>[2x]MTT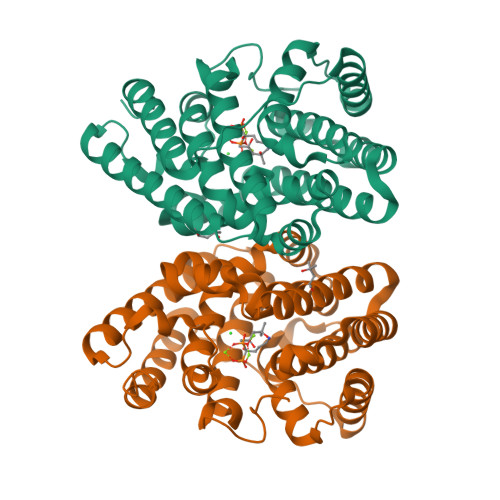GLSTAGAQDIGRSSVRPYLEECTRRFQEMFDRHVVTRPTKVELTDAELREVIDDCNAAVAPLGKTVSDERWISYVGVVLWSQSPRHIKDMEAFKAVCVLNCVTAVWDDMDPALHDFGLFLPQLRKICEKYYGPEDAEVAYEAARAFVTSDHMFRDSPIKAALCTTSPEQYFRFRVTDIGVDFWMKMSYPIYRHPEFTEHAKTSLAARMTTRGLTIVNDFYSYDREVSLGQITNCFRLCDVSDETAFKEFFQARLDDMIEDIECIKAFDQLTQDVFLDLIYGNFVWTTSNKRYKTAVNDVNSRIQAAALEHHHHHH> ISSAIQVGHQLALIGDEFNRAY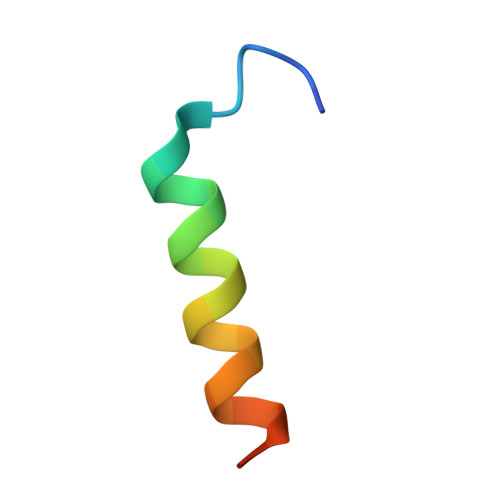SRK2,4-dibromo-6-{[(2-nitrobenzene-1-carbonyl)amino]methyl}phenyl 4-bromobenzoate | C21 H13 Br3 N2 O5 | 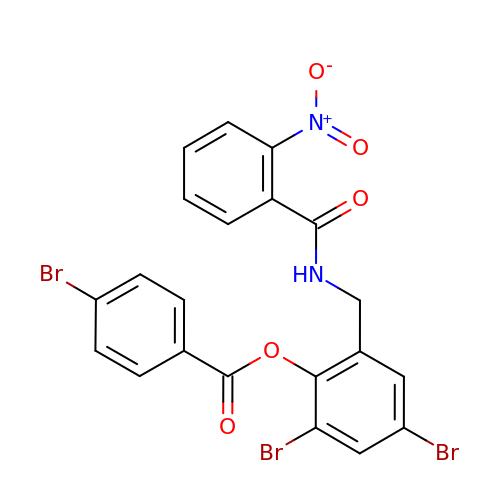KBKZNODCWQTWQF-UHFFFAOYSA-N>[2x]MSE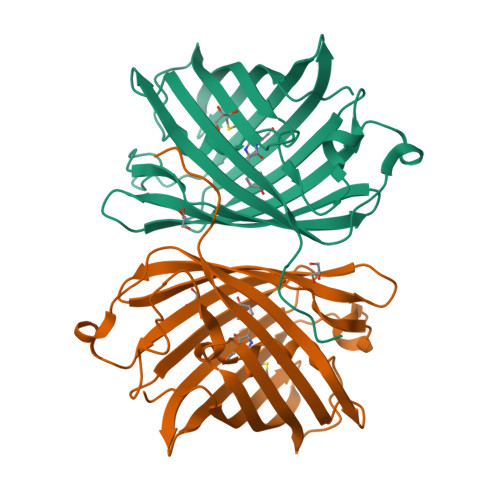LITENMHMKLYMEGTVNNHHFKCTSEGEGKPYEGTQTQRIKVVEGGPLPFAFDILATSFMYGSHTFINHTQGIPDFWKQSFPEGFTWERVTTYEDGGVLTATQDTSLQDGCLIYNVKIRGVNFPSNGPVMQKKTLGWEAHTEMLYPADGGLEGRADLALKLVGGGHLICNFKTTYRSKKPAKNLKMPGVYYVDYRLERIKEADKETYVEQHEVAVARYCDLPSKLGHKLN>MAHHHHHHMSTPQLMRVKKLSEFAILPVRSSQFAAGFDLASAYDYVVPARGKCLVKTDLAVAVPHGYYGRVAPRSGLAVKNFIDVGAGVVDSDYRGNLGVLLFNHGDEDFKIARGDRIAQFVIEQIALPDIVEVDDLDETERGAGGFGSTGV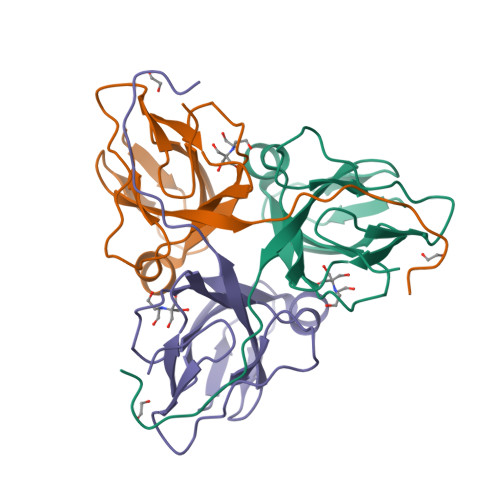KSK[5x]>[12x]GAMTSQINRQYQLAQRPSGLPGRDTFSFVETPLGEPAEGQILVKNEYLSLDPAMRGWMNDARSYIPPVGIGEVMRALGVGKVLVSKHPGFQAGDYVNGALGVQDYFIGEPKGFYKVDPSRAPLPRYLSALGMTGMTAYFALLDVGQPKNGETVVISGAAGAVGSVAGQIARLKGC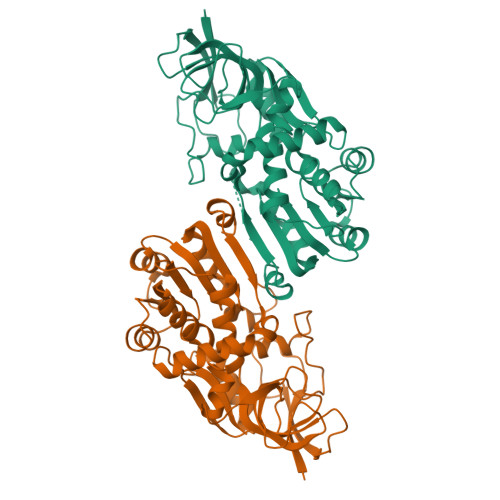RVVGIAGGAEKCRFLVEELGFDGAIDYKNEDLAAGLKRECPKGIDVFFDNVGGEILDTVLTRIAFKARIVLCGAISQYNNKEAVRGPANYLSLLVNRARMEGMVVMDYAQRFPEGLKEMATWLAEGKLQSREDIVEGLETFPETLLKLFSGENFGKLVLKV> LNMKYRKRQLVTREAQIKDWVENELEALKLEA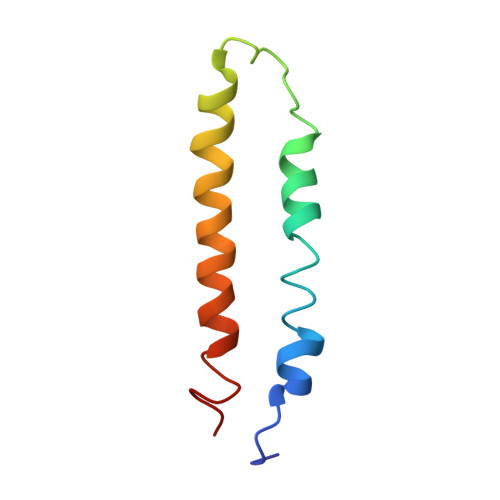EEIPSEDQNEFLLERTREIHNEAESQLRAAQQQWGNDFY BENZOFURAN-2-CARBOXYLIC ACID {(S)-3-METHYL-1-[3-OXO-1-(PYRIDIN-2-YLSULFONYL)AZEPAN-4-YLCARBAMOYL]BUTYL}AMIDE | C26 H30 N4 O6 S | 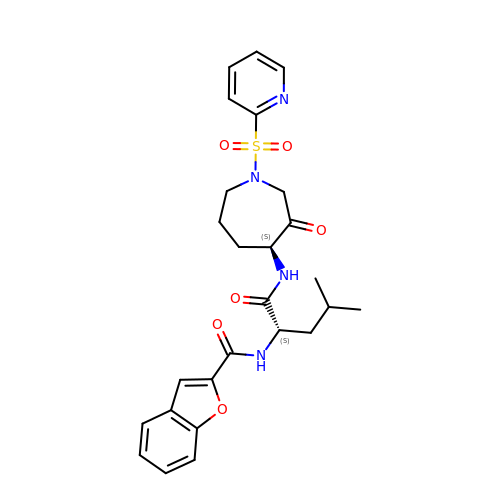VBPPNJCVXGAZDD-PMACEKPBSA-N>ADCAKGKIEFSKYNEDDTFTVKVDGKEYWTSRWNLQPLLLSAQLTGMTVTIKSSTCESGSGFAEVQFNND[10x]

The pathogenesis of E. coli O157:H7 is in large part due to the production of Shiga toxin (Stx), an AB5 toxin that consists of a ribosomal RNA-cleaving A-subunit surrounded by a pentamer of receptor-binding B subunits. There are two major isoforms, Stx1 and Stx2, which differ dramatically in potency despite having 57% sequence identity. The B-pentamer binds to the glycolipid globotriaosylceramide (Gb3) on the surface of host cells and delivers the A-subunit into the cell. Analytical ultracentrifugation using purified B-subunits demonstrates that Stx2B, the more deadly isoform, shows decreased pentamer stability compared to Stx1B (EC50 = 2.3 µM vs. EC50 = 0.043 µM for Stx1B).

Examination of the structures for potentially destabilizing amino acids in the inter-B-subunit interface revealed a notable difference at position 40 of Stx2B, which corresponds to amino acid 41 in Stx1B. Gln40 in Stx2B lies in an otherwise hydrophobic pocket and closely approaches Leu38 (inset). To test the role of L41/Q40 in B-pentamer stability, we generated the reciprocal point mutants Stx1B-L41Q and Stx2B-Q40L. In contrast, the reciprocal mutant Stx2B-Q40L stabilized the inter-B-subunit interaction to the extent that the pentameric species predominated in sedimentation velocity experiments down to 0.5 µM, the detection limit of the absorbance optics. EC50 values, calculated from the K5 values, were 0.043 and 0.106 µM for Stx1B and Stx2B-Q40L, respectively. CD measurements of the ellipticity at 219 nm as a function of temperature revealed that the Q40L mutation raised the Tm of Stx2B by 18°C relative to wild-type Stx2B, whereas the reciprocal mutation L41Q in Stx1B lowered the Tm by at least 15°C relative to wild-type Stx1B (the unfolding transition for Stx1B was not completed by 95°C and thus could not be determined precisely). X-ray crystallographic studies of Stx2B-Q40L were undertaken to gain better insight into molecular packing at the inter-B-subunit interface. As expected based on the CD data, no global structural changes were observed in an overlay of the Cα traces of a single B-subunit of wild-type Stx2B and Stx2B-Q40L (average RMSD  = 0.37 Å). The leucine in the mutant packs well into the hydrophobic pocket of the adjacent subunit, whereas the wild-type glutamine residue appears to be offset from the groove. This confirmed the CD data indicating that the change in solution behavior was not due to any large-scale structural changes, but rather the destabilizing effect of the unfavorable presence of the polar side-chain of Q40 in an otherwise hydrophobic pocket.>MKVWNARNDHLTINQWATRIDEILEAPDGGEVIYNVDENDPREYDAIFIGGGAAGRFGSAYLRAMGGRQLIVDRWPFLGGSCPHNACVPHHLFSDCAAELMLARTFSGQYWFPDMTEKVVGIKEVVDLFRAGRNGPHGIMNFQSKEQLNLEYILNCPAKVIDNHTVEAAGKVFKAKNLILAVGAGPGTLDVPGVNAKGVFDHATLVEELDYEPGSTVVVVGGSKTAVEYGCFFNATGRRTVMLVRTEPLKLIKDNETRAYVLDRMKEQGMEIISGSNVTRIEEDANGRVQAVVAMTPNGEMRIETDFVFLGLGEQPRSAELAKILGLDLGPKGEVLVNEYLQTSV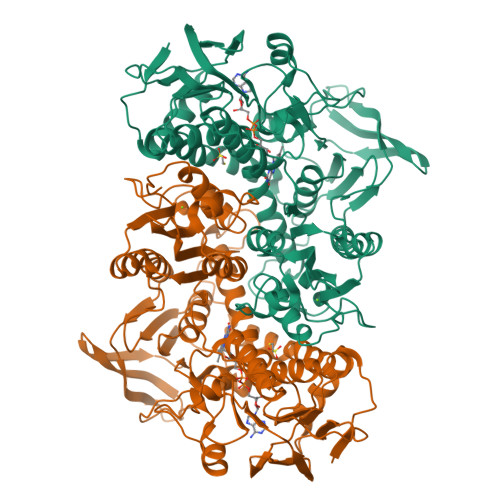PNVYAVGDLIGGPMEMFKARKSGCYAARNVMGEKISYTPKNYPDFLHTHYEVSFLGMGEEEARAAGHEIVTIKMPPDTENGLNVALPASDRTMLYAFGKGTAHMSGFQKIVIDAKTRKVLGAHHVGYGAKDAFQYLNVLIKQGLTVDELGDMDELHLNPTEFIQLSRLRAGSKNLVSL[2x]Chitin is a long-chain polymer of β-(1,4)-linked N-acetylglucosamine (GlcNAc) and is synthesized by chitin synthase in the plasma membrane. In this report, we determined seven cryo-electron microscopy (cryo-EM) structures of S. cerevisiae Chs1 in the apo state and in complex with UDP-GlcNAc, UDP-GlcNAc+GlcNAc, UDP, UDP+GlcNAc, PolyB, and NikkoZ. The overall structure of Chs1 reveals a dimer architecture with a twofold symmetry and is ~100 Å tall and 110 Å wide. Each Chs1 monomer is composed of a large cytosolic soluble region and a transmembrane domain (TMD), with both the N-terminus and C-terminus in the cytosol.

The nucleoside moieties of PolyB and NikkoZ are the same 5-aminohexuronic acid N-glycosidically bound to uracil. In contrast, the peptidyl moieties of PolyB contain carbamoylpolyoxamic acid, and NikkoZ contains hydroxypyridylhomothreonine. We determined the structures of Chs1-PolyB and the Chs1-NikkoZ complex at 3.6-Å and 2.4-Å resolution, respectively. Comparison between Chs1 maps in the apo and inhibitor-bound states revealed clearly elongated extra densities corresponding to PolyB and NikkoZ in the active site, consistent with their function as substrate competitive inhibitors. The nucleoside moieties of PolyB and NikkoZ are stabilized by T453, M454, Y455, and K578 at the top of the active site, which are the same residues interacting with the nucleoside group of UDP-GlcNAc. In contrast, unlike the flexible GlcNAc moiety of UDP-GlcNAc extending away from the active site, the peptidyl moieties of PolyB and NikkoZ extend toward the chitin transport channel and form extensive interactions with E457, D602, A677, and W760. The unique architecture of peptidyl moiety makes the inhibitor locked inside of the active site of Chs1. Besides, the switch loop of Chs1 is open in our Chs1-PolyB and Chs1-NikkoZ structures. Notably, end part of the peptidyl moieties of PolyB and NikkoZ occupy the GlcNAc acceptor binding site, and thus block the chitin transport channel. Therefore, our structures suggest that the peptidyl nucleoside inhibitors inhibit chitin synthases using a unique mechanism: the nucleoside moiety competes with UDP binding, and the peptidyl moiety induces the switch loop open and blocks the gate of chitin transport channel.

>[2x]MSDQNNRSRNEYHSNRKNEPSYELQNAHSGLFHSSNEELTNRNQRYTNQNASMGSFTPVQSLQFPEQSQQTNMLYNGDDGNNNTINDNERDIYGGFVNHHRQRPPPATAEYNDVFNTNSQQLPSEHQYNNVPSYPLPSINVIQTTPELIHNGSQTMATPIERPFFNENDYYYNNRNSRTSPSIASSSDGYADQEARPILEQPNNNMNSGNIPQYHDQPFGYNNGYHGLQAKDYYDDPEGGYIDQRGDDYQINSYLGRNGEMVDPYDYENSLRHMTPMERREYLHDDSRPVNDGKEELDSVKSGYSHRDLGEYDKDDFSRDDEYDDLNTIDKLQFQANGVPASSSVSSIGSKESDIIVSNDNLTANRALKRSGTEIRKFKLWNGNFVFDSPISKTLLDQYATTTENANTLPNEFKFMRYQAVTCEPNQLAEKNFTVRQLKYLTPRETELMLVVTMYNEDHILLGRTLKGIMDNVKYMVKKKNSSTWGPDAWKKIVVCIISDGRSKINERSLALLSSLGCYQDGFAKDEINEKKVAMHVYEHTTMINITNISESEVSLECNQGTVPIQLLFCLKEQNQKKINSHRWAFEGFAELLRPNIVTLLDAGTMPGKDSIYQLWREFRNPNVGGACGEIRTDLGKRFVKLLNPLVASQNFEYKMSNILDKTTESNFGFITVLPGAFSAYRFEAVRGQPLQKYFYGEIMENEGFHFFSSNMYLAEDRILCFEVVTKKNCNWILKYCRSSYASTDVPERVPEFILQRRRWLNGSFFASVYSFCHFYRVWSSGHNIGRKLLLTVEFFYLFFNTLISWFSLSSFFLVFRILTVSIALAYHSAFNVLSVIFLWLYGICTLSTFILSLGNKPKSTEKFYVLTCVIFAVMMIYMIFCSIFMSVKSFQNILKNDTISFEGLITTEAFRDIVISLGSTYCLYLISSIIYLQPWHMLTSFIQYILLSPSYINVLNIYAFCNVHDLSWGTKGAMANPLGKINTTEDGTFKMEVLVSSSEIQANYDKYLKVLNDFDPKSESRPTEPSYDEKKTGYYANVRSLVIIFWVITNFIIVAVVLETGGIADYIAMKSISTDDTLETAKKAEIPLMTSKASIYFNVILWLVALSALIRFIGCSIYMIVRFFKKVTFRGGSGGDYKDDDDKDYKDDDDKDYKDDDDK> MAETSEEVAVLVQRVVKDITNAFRRNPHIDEIGLIPCPEARYNRSPIVLVENKLGVESWCVKFLLPYVHNKLLLYRTRKQWL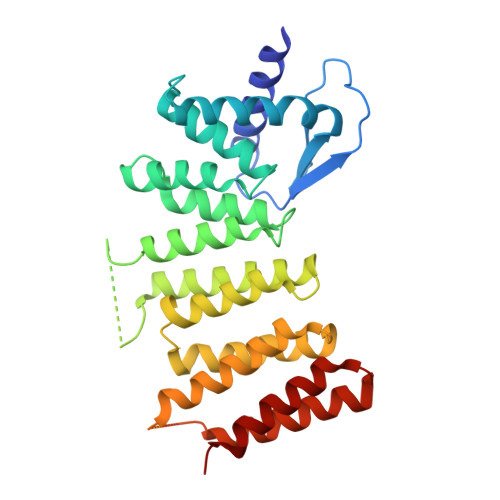NRDELIDVTCTLLLLNPDFTTAWNVRKELILSGTLNPIKDLHLGKLALTKFPKSPETWIHRRWVLQQLIQETSLPSFVTKGNLGTIPTERAQRLIQEEMEVCGEAAGRYPSNYNAWSHRIWVLQHLAKLDVKILLDELSSTKHWASMHVSDHSGFHYRQFLLKSLISQTVIDSSVMEQNPLRSEPALVPPKDEEAAVSTEEPRINLPHLLEEEVEFSTDLIDSYPGHETLWCHRRHIFYLQHHLN> MSQEALKAPVVVL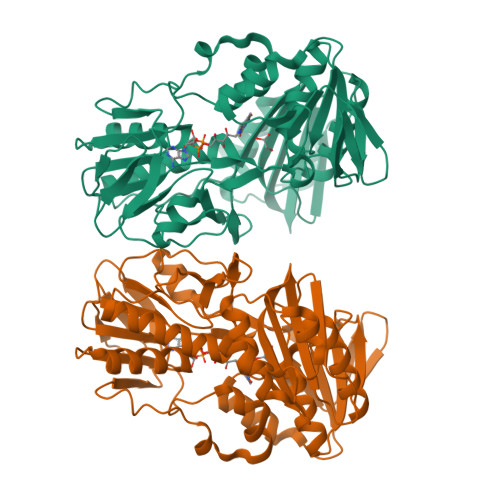GAGLASVSFVAELRQAGYQGLITVVGDEAERPYDRPPLSKDFMAHGDAEKIRLDCKRAPEVEWLLGVTAQSFDPQAHTVALSDGRTLPYGTLVLATGAAPRALPTLQGATMPVHTLRTLEDARRIQAGLRPQSRLLIVGGGVIGLELAATARTAGVHVSLVARGPRLMSRAAPATLADFVARYHAAQGVDLRFERSVTGSVDGVVLLDDGTRIAADMVVVGIGVLANDALARAAGLACDDGIFVDAYGRTTCPDVYALGDVTRQRNPLSGRFERIETWSNAQNQGIAVARHLVDPTAPGYAELPWYWSDQGALRIQVAGLASGDEEIVRGEVSLDAPKFTLIELQKGRIVGATCVNNARDFAPLRRLLAVGAKPDRAALADPATDLRKLAAAVAA> MKKNKKTTKSLLSADEKITESLRSTLSDVLPDQLQTYIRTVLQFSGRPEGANLLTGPNTEIEFFSQDPNKNFPNIFAKYSNVLTVSSDPNFITSEDEEVKIIWGRHGSDSLIGFDPGADLVGKRRIDIFLGDFIDEQFNPIPGALNAGKSWSDRFILGDWQKPYYFEDDETLGLNQSAMILDFNPNEDVIQLHGDRQDYELVNISLGTAIFWREKKGYDLIGVLGGVSDLSLKGDYFEFKGNTAPKTVLKTAEHIGTAANDYIFSSTVDAKGNFYVGGGTGGSLGGRNIGARDAWLAKYDSNGNQRWSRQFGSTGTESLWGMASDGSNIYVAGNTTGQLENNTVKGGNDAYLAKYDSDGNQVWIKQNGTYTLEESYKITVDSSGNIYTAGATFGSLGGPNQNLEQGEVFELPSTDGYVAKFDSNGNQLWVAQFGTITLDDNWGVAADNNGNVFAGGNTKGSFGAKNTGTAGEYDAWLVKLNKDGQTDWVRQFGTPNYDFMWDIETDSLGDIYATGWTLGDLGGKNAGSYDVWLAKYNTNGNQLWIKQFGTSEDDAPFLDGIDIDANDNIFLTGNTNGNLGGANAGSYDAWAAKFDKDGNQLWLKQFGTPDYDTATTVTAVNFGKLYVSGI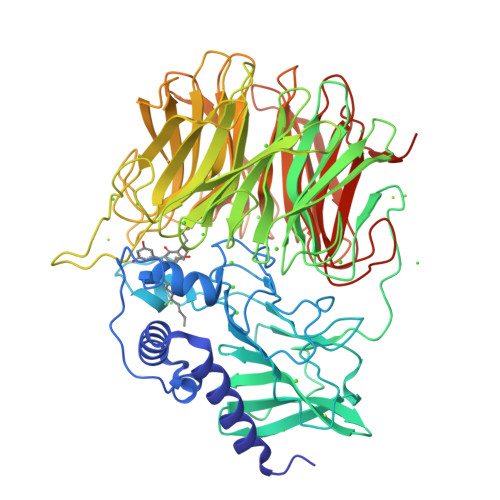TEGSLGTTNAGSYDSWALKLDADNGEIQDFNSSTNTFGQTGFLNLG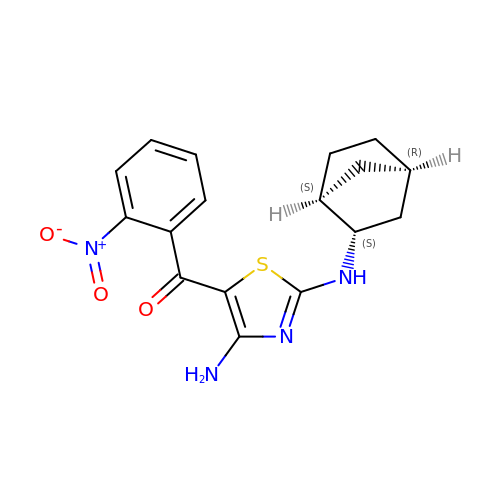(4-amino-2-{[(1S,2S,4R)-bicyclo[2.2.1]heptan-2-yl]amino}-1,3-thiazol-5-yl)(2-nitrophenyl)methanone | C17 H18 N4 O3 S | JRNXAQINDCOHGS-SCVCMEIPSA-N> NQSVVVDFLLPTGVYLNFPVSRNANLSTIKQLLWHRAQYEPLFHMLSGPEAY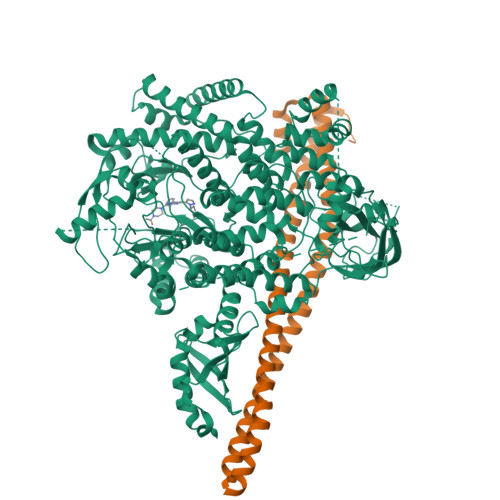VFTCINQTAEQQELEDEQRRLCDVQPFLPVLRLVAREGDRVKKLINSQISLLIGKGLHEFDSLCDPEVNDFRAKMCQFCEEAAARRQQLGWEAWLQYSFPLQLEPSAQTWGPGTLRLPNRALLVNVKFEGSEESFTFQVSTKDVPLALMACALRKKATVFRQPLVEQPEDYTLQVNGRHEYLYGSYPLCQFQYICSCLHSGLTPHLTMVHSSSILAMRDEQSNPAPQVQKPRAKPPPIPAKKPSSVSLWSLEQPFRIELIQGSKVNADERMKLVVQAGLFHGNEMLCKTVSSSEVSVCSEPVWKQRLEFDINICDLPRMARLCFALYAVIEKAKKARSTKKKSKKADCPIAWANLMLFDYKDQLKTGERCLYMWPSVPDEKGELLNPTGTVRSNPNTDSAAALLICLPEVAPHPVYYPALEKILELGRHSECVHVTEEEQLQLREILERRGSGELYEHEKDLVWKLRHEVQEHFPEALARLLLVTKWNKHEDVAQMLYLLCSWPELPVLSALELLDFSFPDCHVGSFAIKSLRKLTDDELFQYLLQLVQVLKYESYLDCELTKFLLDRALANRKIGHFLFWHLRSEMHVPSVALRFGLILEAYCRGSTHHMKVLMKQGEALSKLKALNDFVKLSSQKTPKPQTKELMHLCMRQEAYLEALSHLQSPLDPSTLLAEVCVEQCTFMDSKMKPLWIMYSNEEAGSGGSVGIIFKNGDDLRQDMLTLQMIQLMDVLWKQEGLDLRMTPYGCLPTGDRTGLIEVVLRSDTIANIQLNKSNMAATAAFNKDALLNWLKSKNPGEALDRAIEEFTLSCAGYCVATYVLGIGDRHSDNIMIRESGQLFHIDFGHFLGNFKTKFGINRERVPFILTYDFVHVIQQGKTNNSEKFERFRGYCERAYTILRRHGLLFLHLFALMRAAGLPELSCSKDIQYLKDSLALGKTEEEALKHFRVKFNEALRESWKT;> QQDQVVKEDNIEAVGKKLHEYNTQFQEKSREYDRLYEDYTRTSQEIQMKRTAIEAFNETIKIFEEQCQTQERYSKEYIEKFKREGNETEIQRIMHNYEKLKSRISEIVDSRRRLEEDLKKQAAEYREIDKRMNSIKPDLIQLRKTRDQYLMWLTQKGVRQKKLNEWLG>MRGSHHHHHHGSKKGDLVAWNKENDRRTLWTTPDPSPNCKVSEEKDSKLTLVLTKCGSQILASVSLLVVKGKFANINNKTNPGEDYKKFSVKLLFDANGKLLTGSSLDGNYWNYKNKDSVIGSPYENAVPFMPNSTAYPKIINNGTANPEDKKSAAKKTIVTNVYLGGDAAKPVATTISFNKETESNCVYSITFDFAWNKTYKNVPFDSSSLTFSYIAQDAEDKNE[6x]

Here, we investigated HAdV-D49, which previously has been studied for vaccine and vascular gene transfer applications. Here, we structurally and functionally investigate the tropism of HAdV-D49, focussing on the fiber knob protein as the major mediator of cellular attachment, and evaluate the potential utility of a pseudotyped HAdV-C5/D49K vector to infect a range of cancer cell lines. We investigated the tropism of HAdV-D49, demonstrating it uses a novel cell entry mechanism that bypasses all known HAdV receptors. We demonstrate HAdV-D49 fiber knob has weak affinity for CAR, although it is not dependent upon this interaction to mediate efficient cell entry, and in fact the presence of CAR may even inhibit cellular transduction.

To investigate other closely related HAdV with homologous fiber-knob proteins we performed a BLASTp search using the HAdV-D49K amino acid sequence. This search revealed that the HAdV-D30K protein is highly homologous to HAdV-D49K, differing in just 4 amino acid residues ([Fig fig4]). Residue 338 is not surface exposed on either fiber knob protein and is likely to be functionally homologous (HAdV-D49 = Isoleucine338, HAdV-D30 = Valine338). However, the remaining 3 residue differences, E339K, G331A, and Q332K (HAdV-D30K → D49K) are surface exposed at the apex of each fiber knob monomer ([Fig fig4]). We further investigated the effect of the opposing charges at residue substitutions 339 and 332 ([Fig fig4]) by modelling the electrostatic surface potential of the two fiber knob proteins, based on our crystal structures ([Fig fig5]). The surface potential maps reveal that whilst structural homology was high, they present radically different electrostatic surface potential distributions. HAdV-D30K is significantly more acidic (pI = 5.57) than HAdV-D49K (pI = 8.26) ([Fig fig5]). HAdV-D49K can be seen to have much more basic potential around the apex where the residue substitutions are. Thus, it seems probable that the interaction requires the basic electrostatic potential. Structurally and biologically we demonstrate that HAdV-D49 knob protein is unable to engage CD46, whilst potential interaction with CAR is extremely limited by extension of the DG loop.> MEINPYLLMLNNDITSMISLTYPYTGAPPMSHGTSTKYSMETVSRTYSYSRTKKEVPSGIFPIERRKFCNTIEDKENLEKPNGNVDINFMLSLAEMLEEKMGKGFFKFCANEAEAEILKMHFSKLTEGRQTYDWTSERNMPAATALQLTVDAIQETQGTFKGTTMVEYCNKILEMMDWPEVKFKKVRMIVQRHWDPKTKKEIKMKSPTLMITKIGREEFIKRICTINTMAKDGERGKYKRRAIATPGMGIRPFSKIVETLAQKICERLAESGLPVGGNEKKAKLKTTVSSTNSKLQEGQFMVNITGDNSKWNECQQPEAYLAMLAYITKDSSNLMKDLCSVAPTLFCNKYVKMGQGFRAKNKRKTKEIVIPAKKMKERKELMNAEWRDLFETIEPYMDGECCFLGGGMLMGMFNMLSTVFGVMTLNYREEALARRNCYWTGLQSSDDFVLFCISRTWPEMEMTILKFIAVCKLMGINMSLEKSYGCLPELFEFTSMFFSGDFVSNIALELPAFTTAGMNEGTDFTAAMSVIRTNMINNGLSPGTALMALRICLQEFRATYRVHPYDSGVKNHRMKIIRKFIETIENK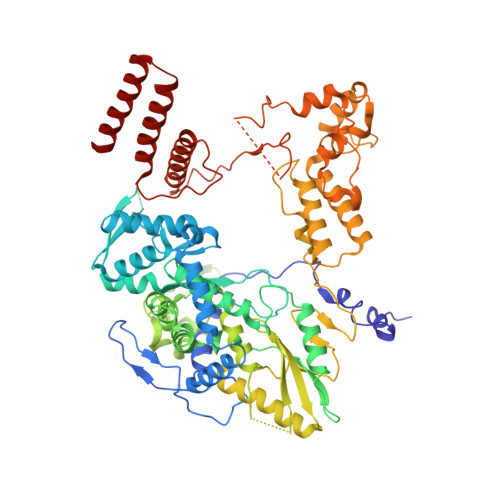DGLLISDGGKLMNNISSLHIPEEILKEDLMDPSYRNRVFNPRNPFTQFEKTVDIFKASGPIRVEENEAVVSTHSFRTRSNRTLLNTDMRAMALEEKRYQVVCNMYRSVFESADVNTPIGSMSMGEAIEAKILDRARTQFENGIIGGEEYSEIKRLIEDAKRQRLSV>DRHHHHHHKLSPANDDQSRPSLSNGHTCVGCVLVVSVIEQLAQVHNSTVQASMERLCSYLPEKLFLKTTCYLVIDKFGSDIIKLLSADMNADVVCHTLEFCKQNTGQPLCHLYPLPKETWKFTLQKARQIVKKSPILKY[2x];>[2x]SRSGSDICSLPVLAKICQKIKLAMEQSVPFKDVDSDKYSVFPTLRGYHWRGRDCNDSDESVYPGRRPNNWDVHQDSNCNGIWGVDPKDGVPYEKKFCEGSQPRGIILLGDAAGAHFHISPEWITASQMSLNSFINLPTALTNELDWPQLSGATGFLDSTVGIKEKSIYLRLWKRNHCNHRDYQNISRNGASSRNLKKFIESLSRNKVLDYPAIVIYAMIGNDVC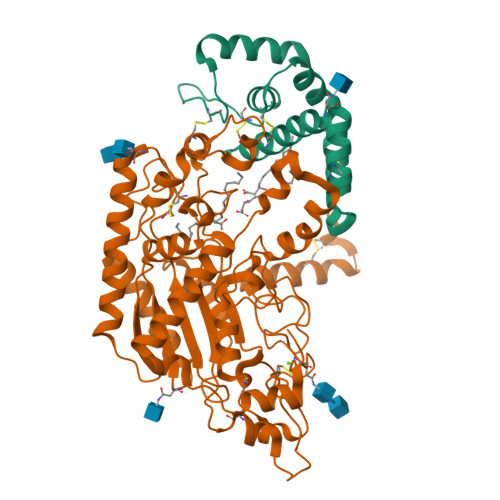SGKSDPVPAMTTPEKLYSNVMQTLKHLNSHLPNGSHVILYGLPDGTFLWDNLHNRYHPLGQLNKDMTYAQLYSFLNCLQVSPCHGWMSSNKTLRTLTSERAEQLSNTLKKIAASEKFTNFNLFYMDFAFHEIIQEWQKRGGQPWQLIEPVDGFHPNEVALLLLADHFWKKVQLQWPQILGKENPFNPQIKQVFGDQGGH> GMAYTTTVKLDGDTKTYTLSPTVKKYTLMDLGFVKGRSGAFSFERSLDPTSPYQAAFKLKMTVNADLTGFKMTTVTGNGVQRANIFKNDAHPEAVEQLRYILANFIERDILTTD

The structure of LP2179, a member of the PF08866 (DUF1831) family, suggests a novel α+β fold comprising two β-sheets packed against a single helix. The LP2179 gene of Lactobacillus plantarum, a lactic acid-producing bacterium found in human saliva and intestinal flora, encodes a protein with a molecular weight of 12.6 kDa (residues 1–113) and a calculated isoelectric point of 8.9. A remote structural similarity to two other uncharacterized protein families specific to the Bacillus genus (PF08868 and PF08968), as well as to prokaryotic S-adenosylmethionine decarboxylases, is consistent with a role in amino-acid metabolism. Genomic neighborhood analysis of LP2179 supports this functional assignment, which might also then be extended to PF08868 and PF08968.

The final model includes 114 residues (i.e. the residual Gly0 from the expression tag followed by residues 1–113 of LP2179), one glycerol molecule, one chloride ion and 195 water molecules in the asymmetric unit. The side chains of Lys8, Lys59 and Lys86 were not modeled owing to poor electron density. The Ramachandran plot produced by MolProbity shows that 98.2% and 100% of the residues are in favored and in favored and additionally allowed regions, respectively. LP2179 forms a single domain composed of two antiparallel β-­sheets packed against a long C-terminal helix H3. A second helix, H1, links strand β2 from the first β-sheet (order 127), which is assembled from the two N-terminal and the C-terminal β-strands, to the second β-sheet (order 3456) and packs parallel to H3. Analysis of the crystallographic packing of LP2179 using the PISA server and analytical size-exclusion chromatography in combination with static light scattering indicate that a monomer is the likely quaternary form. The H2 helix, which is absent in both YugN-like and DUF1885 homologs, might constitute an additional difference, but owing to its short size (one helical turn) and its involvement in crystal contacts (Asp88–Arg107′ and Phe85–Arg107′) it might not represent a biologically relevant conformation of this region in solution. Among these TBP-like variants, LP2179 is unique in that the N- and C-terminal β-strands are combined to form an additional β-sheet that is situated between the central β-sheet and helix H3. In LP2179, a strand is added at both the N- and C-termini, while YugN-like homologs contain an extra β-strand at the N-terminus (topology β2-α-β4-α) and PF08968 homologs contain an additional β-strand at the C-terminus that follows a circular permutation of the core fold (topology α-β4-α-β2). Although the catalytic residues (Ser and Glu) of the AdoMetDC proenzyme are not conserved in LP2179 and YugN-like or Pfam08968 homologs, sequence alignment reveals the conservation of charged and aromatic residue clusters between LP2179 and YugN-like homologs.> MPDFLGHAENPLREEEWARLNETVIQVARRSLVGRRILDIYGPLGAGVQTVPYDEFQGVSPGAVDIVGEQETAMVFTDARKFKTIPIIYKDFLLHWRDIEAARTHNMPLDVSAAAGAAALCAQQEDELIFYGDA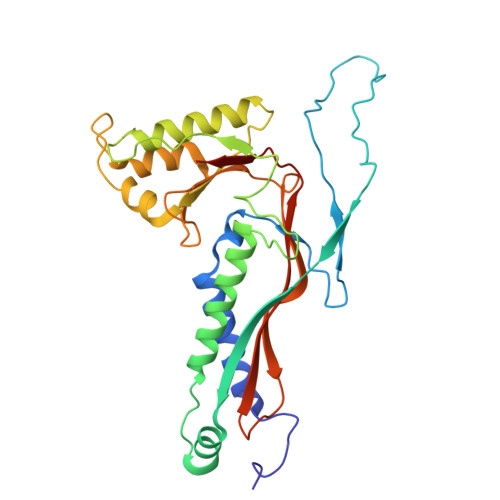RLGYEGLMTANGRLTVPLGDWTSPGGGFQAIVEATRKLNEQGHFGPYAVVLSPRLYSQLHRIYEKTGVLEIETIRQLASDGVYQSNRLRGESGVVVSTGRENMDLAVSMDMVAAYLGASRMNHPFRVLEALLLRIKHPDAICTLEGAGATERR HEXAN-1-OL | 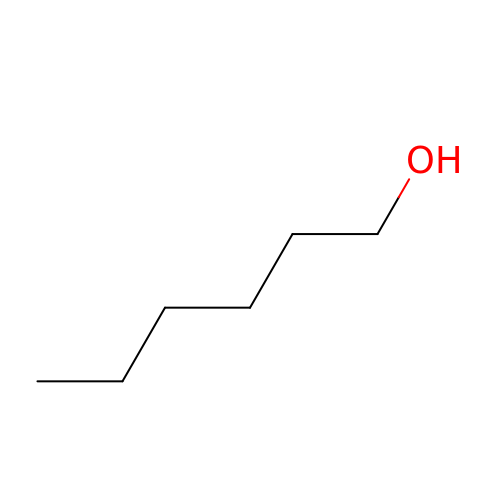C6 H14 O | ZSIAUFGUXNUGDI-UHFFFAOYSA-N>MKMLLIHSDYLEFEAKEKTKIAEETENLKGKLDECLACFIAVEREDENNPEGTAIGAVEEIEKVANQLKVNNIVVYPYAHLSSDLSSPETAVKVLKDIESILKERGYNVLRAPFGWYKAFKISCKGHPLSELSRKIVAKE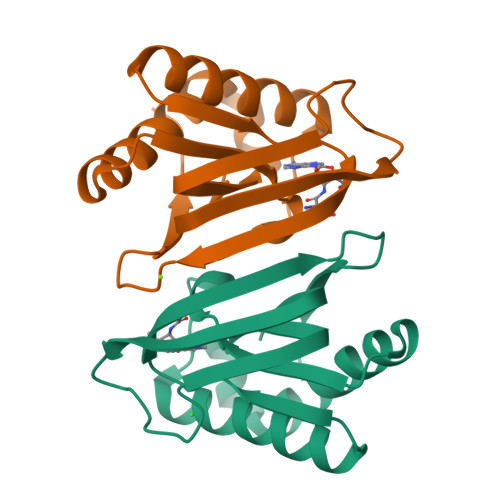E[6x]(Z,2R,4S)-1-(4-methoxy-5-methylidene-2-oxidanylidene-furan-3-yl)-2,4-dimethyl-dodec-6-ene-1,5-dione 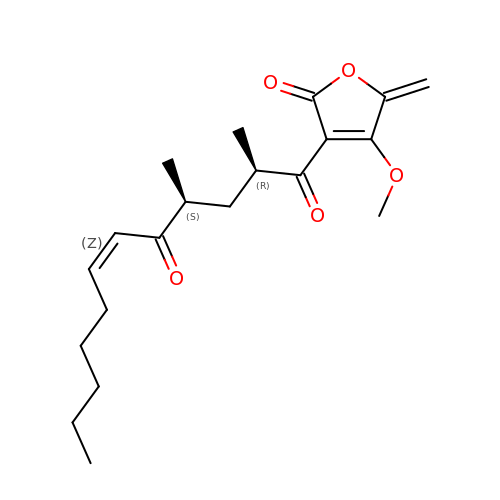| C20 H28 O5 | YWDTUXUXYXSRKL-UONOGXRCSA-N>[4x]PMTL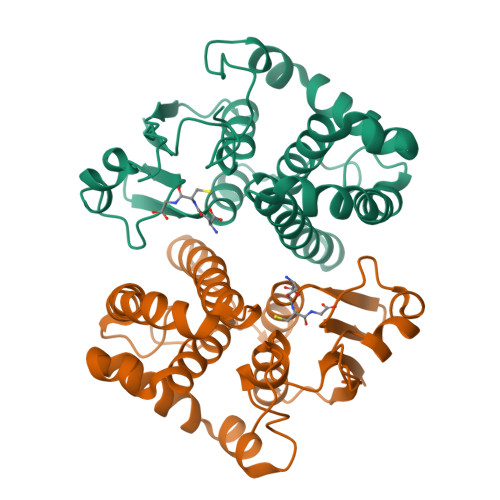GYWNIRGLAHSIRLLLEYTDSSYEEKKYTMGDAPDYDRSQWLNEKFKLGLDFPNLPYLIDGTHKITQSNAILRYIARKHNLCGESEKEQIREDILENQFMDSRMQLAKLCYDPDFEKLKPEYLQALPEMLKLYSQFLGKQPWFLGDKITFVDFIAYDVLERNQVFEPSCLDAFPNLKDFISRFEGLEKISAYMKSSRFLPRPVFTKMAVFGNK> MRRSFLKTIGLGVIALFLGLLNPLSAASYPPIKNTKVGLALSSHPLASEIGQKVLEEGGNAIDAAVAIGFALAVVHPAAGNIGGGGFAVIHLANGENVALDFREKAPLKATKNMFLDKQGNVVPKLSEDGYLAAGVPGTVAGMEAMLKKYGTKKLSQLIDPAIKLAENGYAISQRQAETLKEARERFLKYSSSKKYFFKKGHLDYQEGDLFVQKDLAKTLNQIKTLGAKGFYQGQVAELIEKDMKKNGGIITKEDLASYNVKWRKPVVGSYRGYKIISMSPPSSGGTHLIQILNVMENADLSAL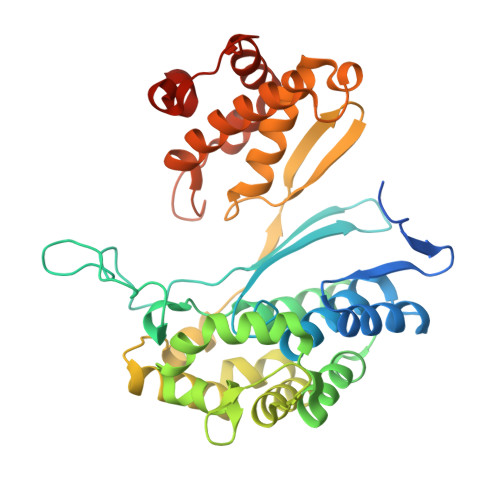GYGASKNIHIAAEAMRQAYADRSVYMGDADFVSVPVDKLINKAYAKKIFDTIQPDTVTPSSQIKPGMGQLHEGSN>MSIRDEALLVGTKVTTKAGDKNIENITLEDEVLQFDMNTKDFSYTNPTKTQKVIRDEIYHFEGAGFDQKVSPNHRMIYEQGGEIKECLAKDFEPSEDKYFIIVEGSHMQIKRIKSTDVKITHTKLDEPTEFHALSVPGKSFVVTDEHGNRSVTGASMHVEGKLGG[2x]

Inteins (intervening proteins) are protein domains inserted into host proteins that are found in all domains of life. They remove themselves out of their precursor proteins in an autocatalytic process called protein splicing, in which the flanking N‐ and C‐terminal exteins are ligated to form the mature host protein. The more recently discovered and less well‐studied class 3 inteins, by contrast, form an internally branched intermediate in the first step of the pathway. The internal motif C2 : 4 cysteine performs a nucleophilic attack at the N‐scissile bond to give the branched thioester intermediate.

To increase the chances of capturing the intein with active site residues in relevant conformations for splicing we decided to crystallize the precursor and fused the AceL NrdHF fragments with inactivating C124A and N146A mutations. Five native flanking extein residues were included at the N‐ and C‐terminal sides, respectively. Expression of the fused intein domain in E. coli without the inactivating mutations resulted in quantitative splicing with no detectable precursor protein remaining, thus suggesting that the artificial cis‐arrangement did not have an impact on folding and function. We determined the structure of the AceL NrdHF precursor at a resolution of 1.9 Å (see Figures S3 and S4 and Table S2 for sample preparation and general crystal data). The intein adopted the typical HINT fold with the expected localization of the conserved motifs in and around the active site. The asymmetric unit contained two protein chains that form an inter‐chain antiparallel β‐sheet involving residues A12–K15 and come in close proximity at residues E140–G142. Electron density can be observed only for the two N‐ and two C‐terminally flanking residues in chain A as well as two N‐ and three C‐terminal extein residues in chain B, suggesting that extein residues further outside were disordered. All intein residues showed electron density including the three residues (GSH) that were inserted upon fusion of the IntN and IntC fragments. Cys124, in the structure mutated to alanine, was indeed located in the active site at the expected position within the motif C2 motif to allow interactions with both splice junctions and to act as the branch point residue. The distance of the thiol side chain to the carbonyl carbon of the N‐scissile bond would be only 3.0 Å, sufficiently short to trigger the initial N−S acyl transfer without additional larger conformation changes. Our crystal structure shows the M70 side chain centrally located in the hydrophobic core as expected.Collinone | 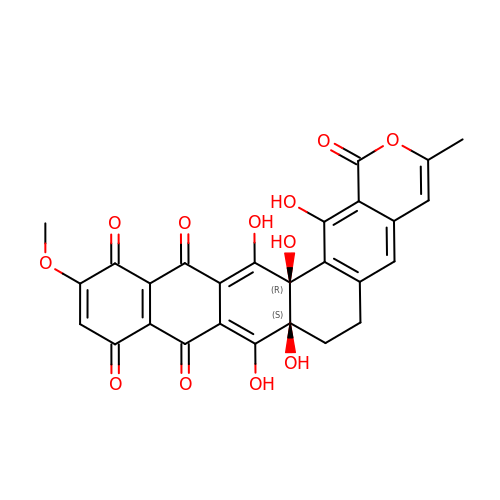C27 H18 O12 | RIDFNHJMBSRPNA-RRPNLBNLSA-N> MFCEKAMELIRELHRAPEGQLPAFNEDGLRQVLEEMKALYEQNQSDVNEAKSGGRSDLIPTIKFRHCSLLRNRRCTVAYLYDRLLRIRALRWEYGSILPNAL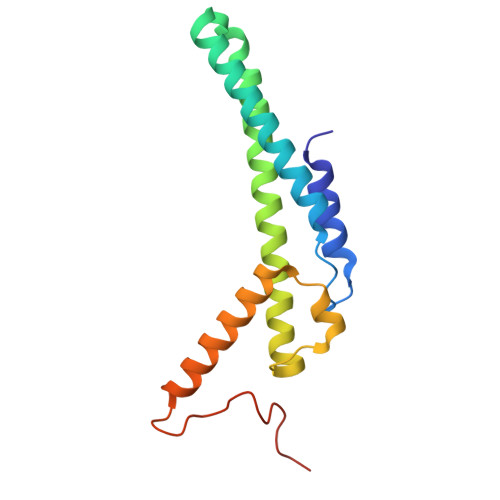RFHMAAEEMEWFNNYKRSLATYMRSLGGDEGLDITQDMKPPKSLYIEVR As a model biocatalyst class, we selected carbamoylases, which promote the hydrolytic cleavage of N‐carbamoyl‐amino acids. Together with hydantoinases, they make up a scalable and widely‐employed enzymatic cascade for the production of enantiopure (un)natural amino acids (=hydantoin process). Based on its reportedly moderate activity for N‐carbamoylated‐ l ‐tyrosine, we produced and purified SmLcar, a carbamoylase from Sinorhizobium meliloti strain CECT 4114. Using this artificial link between enzyme activity and bacterial proliferation, we evolved the carbamoylase SmLcar to accept carbamoylated m‐substituted tyrosine analogs.

When challenged with the synthetic ncAA precursor N‐carbamoyl‐ l ‐3nY (cam‐3nY, 2 mM), SmLcar (10 μM) yielded 6.1 % of the ncAA after 24 hours at pH 6. Conversely, N‐carbamoyl‐ l ‐3iY (cam‐3iY) proved a more challenging substrate, with SmLcar failing to yield detectable levels of 3iY at pH 6 and only providing 0.8 % of the ncAA at pH 8 under otherwise identical conditions. As expected, the parent enzyme displayed a low turnover frequency (k cat=1.05×10−4±1.01×10−5 s−1) and catalytic proficiency (k cat/K M=3.54±0.98×10−2 M−1 s−1). To rationalize the massive performance improvements of our engineered carbamoylases, we obtained crystal structures for SmLcar and the double mutant SmLcar_GC. Guided by the electron densities of unknown small molecules bound to the active sites of SmLcar and SmLcar_GC, we performed docking studies (YASARA) with the synthetic precursor, cam‐3iY, for both enzymes. Comparing the resulting structures of the wild‐type and the evolved variant revealed a striking difference in the orientation of the substrate in their respective binding pockets.

>[2x]MGSSHHHHHHGSGLVPRGSAGMAAPGENRRVNADRLWDSLMEMAKIGPGVAGGNNRQTLTDADGEGRRLFQSWCEEAGLSMGVDKMGTMFLTRPGTDPDALPVHIGSHLDTQPTGGKFDGVLGVLSGLEAVRTMNDLGIKTKHPIVVTNWTNEEGARFAPAMLASGVFAGVHTLEYAYARKDPEGKSFGDELKRIGWLGDEEVGARKMHAYFEYHIEQGPILEAENKQIGVVTHCQGLWWLEFTLTGREAHTGSTPMDMRVNAGLAMARILEMVQTVAMENQPGAVGGVGQMFFSPNSRNVLPGKVVFTVDIRSPDQAKLDGMRARIEAEAPKICERLGVGCSIEAVGHFDPVTFDPKLVETVRGAAEKLGYSHMNLVSGAGHDACWAAKVAPTTMIMCPCVGGLSHNEAEDISREWAAAGADVLFHAVLETAEIVE> MIKQRTLKNIIRATGVGLHSGEKVYLTLKPAPVDTGIVFSRTDLDPVVEIPARAENVGETTMSTTLVKGDVKVDTVEHLLSAMAGLGIDNAYVELSASEVPIMDGSAGPFVFLIQSAGLQEQEAAKKFIRIKREVSVEEGDKRAVFVPFDGFKVSFEIDFDHPVFRGRTQQASVDFSSTSFVKEVSRARTFGFMRDIEYLRSQNLALGGSVENAIVVDENRVLNEDGLRYEDEFVKHKILDAIGDLYLLGNSLIGEFRGFKSGHALNNQLLRTLIA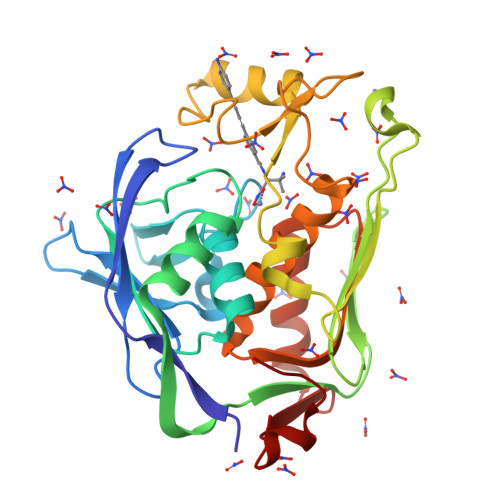DKDAWEVVTFEDARTAPISYMRP> MNFFEYCISTYAKIFEETMNAVGDERVSQKKAIRDTMISAMREFPNVEAAEIWKAVYSAHMDRKSGIADPDIIQKVISAENSWKKSSGHAFEEMIKLLGNSSLEEYGMRILLQKDLNMMIENQEIANEPRDINWLKEQISSNVFDLYITVRNNDKEYVFGCIQSKTSIRDRVTRDREPSMKAMEAFFWSVAICLDGDFLKMPKFIAMVNGGTSNYRLNGWHGMYVFWDKPTIDRIYPIDINLELFVQHAREAAEDWLHRRQWFNYEWKAGQK

To understand how different sequence specificities are achieved within the CCGG-family of restriction endonucleases, we have focused on structural and functional characterization of the BsaWI restriction endonuclease from the thermophilic bacterium Bacillus stearothermophilus W1718. BsaWI recognizes a hexanucleotide 5′-W/CCGGW-3 sequence that accommodates W (A and T) nucleotides outside the CCGG core but rejects S (G and C) nucleotides. The BsaWI protein is folded into two domains: the N-terminal helical domain composed of α helices H1-H3 (residues 1–69; termed N-domain) and the C-terminal catalytic domain (residues 70–272; termed C-domain). We show that in solution BsaWI protein exists in a dimer-tetramer-oligomer equilibrium, but in the presence of specific DNA forms a tetramer bound to two target sites.

The asymmetric unit contains one protein and one DNA chain; a dimer can be generated by rotating protein–DNA chains by the crystallographic two-fold axis. BsaWI forms a stable dimer by swapping the N-domains, while the C-domains are located apart of each other. In the crystal BsaWI forms a dimer in an ‘open’ configuration that approaches the DNA molecule from the minor groove side and makes no sequence specific contacts to DNA bases in the major groove; therefore we term this complex a pre-specific complex. Direct and water-mediated contacts to seven backbone phosphates of each DNA strand are made by eleven residues from each subunit, mostly from the N-domain and from the H4 helix. Two residues of each BsaWI subunit interact with the symmetry related CC:GG half-sites of the recognition sequence. Additionally, K85 contacts the N3 atom of the outer adenine A5 of the same half-site. In the structure of the pre-specific complex these residues are disordered, however the position of the modeled backbone atoms corresponds to the R-(D/E)R residues of NgoMIV in the superimposed structures suggesting that in the specific complex they would make similar contacts to the recognition sequence. Despite the presence of Ca2+ ions in the crystallization buffer there is no electron density that could be interpreted as Ca2+ ion in the vicinity of the active site of BsaWI. In the crystal structure, the BsaWI primary dimers form a linear chain of protein molecules via C-domain contacts. We hypothesize that in the crystal BsaWI primary dimer is an ‘open’ configuration because the crystal contacts at the C-domain interfere with the C-terminal domain closure and transition to the ‘closed’ form observed in EcoRII-C, Ecl18kI, PspGI and BsoBI DNA complexes.> XQARSDIEKLKEAIRDTNKAVQSVQSSIGNLIVAIK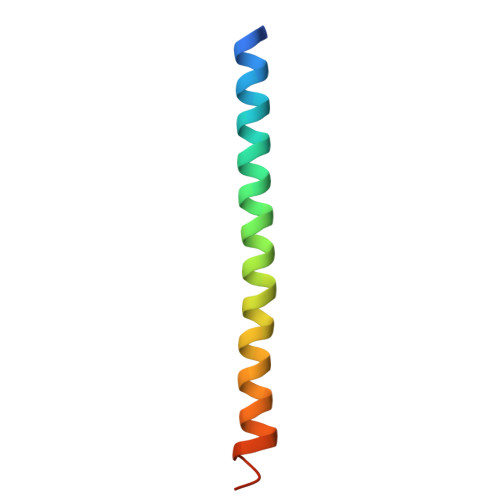SVQDYVNKEIVPSIARX>NLFQFGDMILQKTGKEAVHSYAIYGCYCGWGGQGRAQDATDRCCFAQDCCYGRNLVCNPKTATYTYSFENGDIVCGDNDLCLRAVCECDRAAAICLGENVNTYDKNYEYYSISHC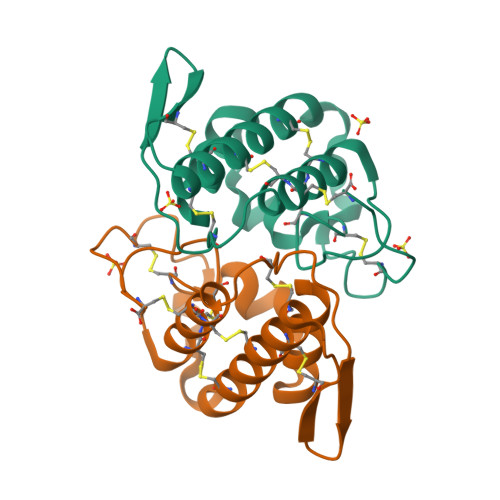TEESEQC[2x]> MGAFTSFVLMLLFTGIILIATNELTYNRP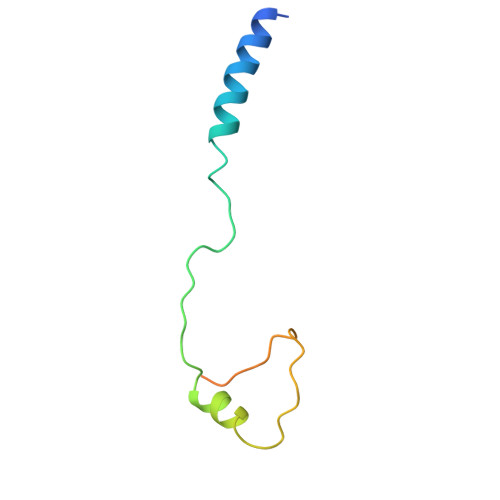REIQYRYLPRDLDSFIRTQEMPSAIFSSMWDVDTRRGGDGGPNPPGIRQSN>MFMREIELRGHIIDSLILPKVFDKILDMGGDYKVLEFEIGKRKTDPSYAKILVIGRDERHVDEILNELRDLGAEIPEIEEVELQPAEKDMVLPE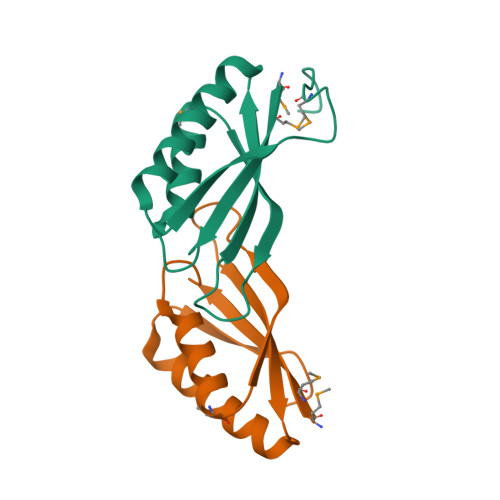GFYSTTNHKTFIRFKGLEHHHHHH[2x]>GHMKQSHFFAHLSRLKLINRWPLMRNVRTENVSEHSLQVAMVAHALAAIKNRKFGGNVNAERIALLAMYHDASEVLTGDLPTPVKYFNSQIAQEYKAIEKIAQQKLVDMVPEELRDIFAPLIDEHAYSDEEKSLVKQADALCAYLKCLEELAAGNNEFLLAKTRLEATLEARRSQEMDYFMEIFVPSFHLSLDEISQDSPL[2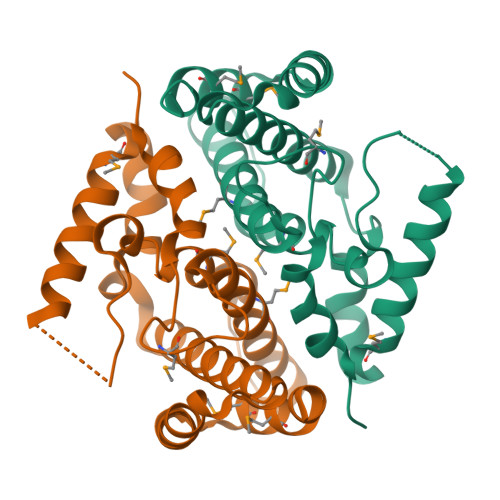x]> SMYVIRDE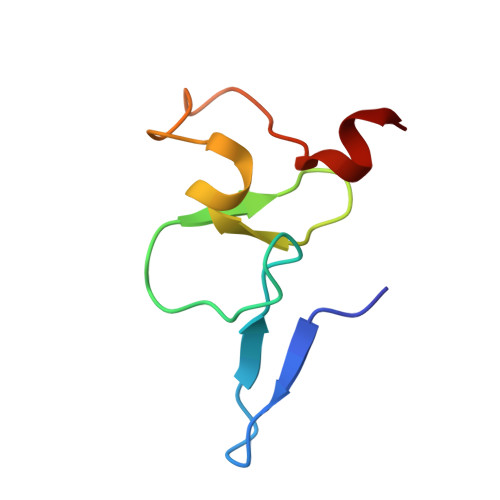WGNQIWICPGCNKPDDGSPMIGCDDCDDWYHWPCVGIMTAPPEEMQWFCPKCANK>[2x]APDTSVSNKQNFSTDVIYQIFTDRFSDGNPANNPTGAAFDGSCTNLRLYCGGDWQGIINKINDG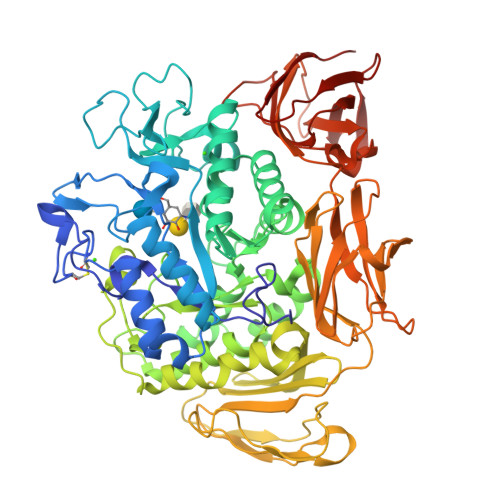YLTGMGITAIWISQPVENIYSVINYSGVNNTAYHGYWARDFKKTNPAYGTMQDFKNLIDTAHAHNIKVIIDFAPNHTSPASSDDPSFAENGRLYDNGNLLGGYTNDTQNLFHHYGGTDFSTIENGIYKNLYDLADLNHNNSSVDVYLKDAIKMWLDLGVDGIRVDAVKHMPFGWQKSFMATINNYKPVFTFGEWFLGVNEISPEYHQFANESGMSLLDLRFAQKARQVFRDNTDNMYGLKAMLEGSEVDYAQVNDQVTFIDNHDMERFHTSNGDRRKLEQALAFTLTSRGVPAIYYGSEQYMSGGNDPDNRARLPSFSTTTTAYQVIQKLAPLRKSNPAIAYGSTHERWINNDVIIYERKFGNNVAVVAINRNMNTPASITGLVTSLPRGSYNDVLGGILNGNTLTVGAGGAASNFTLAPGGTAVWQYTTDATTPIIGNVGPMMAKPGVTITIDGRGFGSGKGTVYFGTTAVTGADIVAWEDTQIQVKIPAVPGGIYDIRVANAAGAASNIYDNFEVLTGDQVTVRFVINNATTALGQNVFLTGNVSELGNWDPNNAIGPMYNQVVYQYPTWYYDVSVPAGQTIEFKFLKKQGSTVTWEGGANRTFTTPTSGTATVNVNWQP> GAV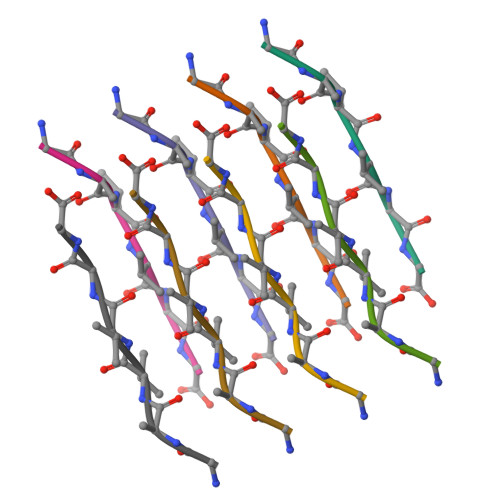VGG3-(5'-{[3,4-bis(hydroxymethyl)benzyl]oxy}-2'-methyl-2-propylbiphenyl-4-yl)pentan-3-ol | C30 H38 O4 | 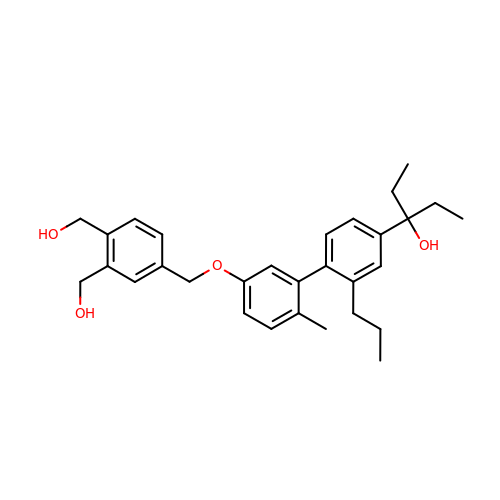RQEWKYJOEHTLIM-UHFFFAOYSA-N> EVRRILPADIKREVLIKDENAETNPDWGFPPEKRPIEMHIQFGVINLDKPPGPTSHEVVAWIKKILNLEKAGHGGTLAPKVSGVLPVALEKATRVVQALLPAGKEYVALMHLHGDVPEDKIIQVMKEFEGEIIQRPPLRSAVKRRLRTRKVYYIEVLEIEGRDVLFRVGVEAGTYIRSLIHHIGLALGVGAHMSELRRTRSGPFKEDETLITLHDLVDYYYFWKEDGIEEYFRKAIQPMEKAVEHLPKVWIKDSAVAAVTHGADLAVPGIAKLHAGIKRGDLVAIMTLKDEL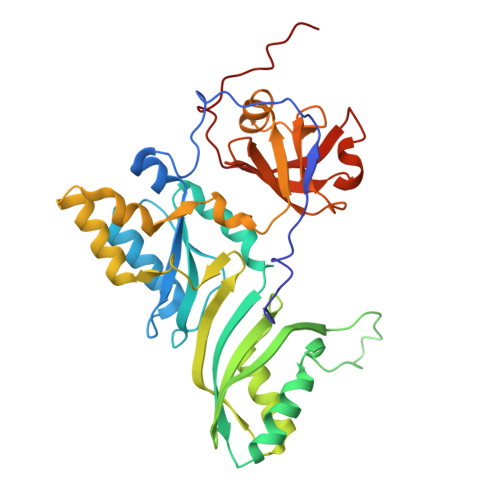VALGKAMMTSQEMLEKTKGIAVDVEKVFMPRDWYPKLWEKRD Cinnamtannin B1 | C45 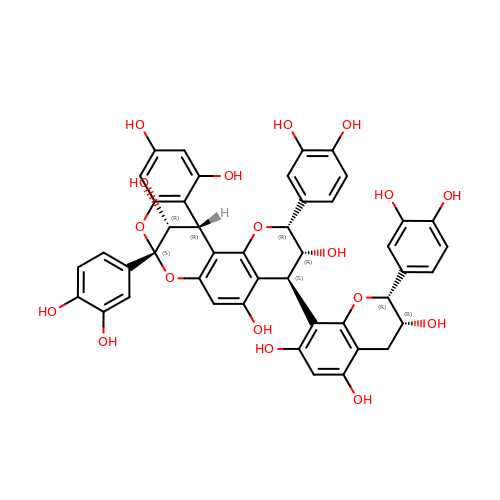H36 O18 | BYSRPHRKESMCPO-LQNPQWRQSA-N> DKMDYDFKVKLSSERERVEDLFEYEGCKVGRGTYGHVYKAKRKDGKDDKDYALKQIEGTGISMSACREIALLRELKHPNVISLQKVFLSHADRKVWLLFDYAEHDLWHIIKFHRASKANKKPVQLPRGMVKSLLYQILDGIHYLHANWVLHRDLKPANILVMGEGPERGRVKIADMGFARLFNSPLKPLADLDPVVVTFWYRAPELLLGARHYTKAIDIWAIGCIFAELLTSEPIFHCRQEDIKTSNPYHHDQLDRIFNVMGFPADKDWEDIKKMPEHSTLMKDFRRNTYTNCSLIKYMEKHKVKPDSKAFHLLQKLLTMDPIKRITSEQAMQDPYFLEDPLPTSDVFAGCQIPYPKREFLTEEEPPLKK;> DKAMAGNFWQSSHYLQWILDKQDLLKERQKDLKFLSEEEYWKLQIFFTNVIQALGEHLKLRQQVIATATVYFKRFYARYSLKSIDPVLMAPTCVFLASKVEEFGVVSNTRLIAAATSVLKTRFSYAFPKEFPYRMNHILECEFYLLELMDCCLIVYHPYRPLLQYVQDMGQEDMLLPLAWRIVNDTYRTDLCLLYPPFMIALACLHVACVVQQKDARQWFAELSVDMEKILEIIRVILKL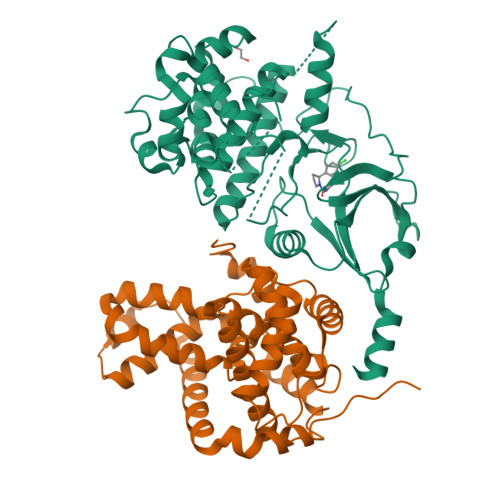YEQWKNFDERKEMATILSKMPKPKPPP>[2x]MRRETVGEFSSDDDDDILLELGTRPPRFTQIPPSSAALQTQIPTTLEVTTTTLNNKQSKNDNQLVNQLNKAQGEASMLRDKINFLNIEREKEKNIQAVKVNELQVKHLQELAKLKQELQKLEDEKKFLQMEARGKSKREVITNVKPPSTTLSTNTNTITPDSSSVAIEAKPQSPQSKKRKISDNLLKKNMVPLNPNRIIPDETSLFLESILLHQIIGADLSTIEILNRLKLDYITEFKFKNFVIAKGAPIGKSIVSLLLRCKKTLTLDRFIDTLLEDIAVLIKEISVHPNESKLAVPFLVALMYQIVQFRPSATHNLALKDCFLFICDLIRIYHHVLKVPIHESNMNLHVEPQIFQYELIDYLIISYSFDLLEGILRVLQSHPKQTYMEFFDENILKSFEFVYKLALTISYKPMVNVIFSAVEVVNIITSIILNMDNSSDLKSLISGSWWRDCITRLYALLEKEIKSGDVYNENVDTTTLHMSKYHDFFGLIRNIGDNELGGLISKLIYTDRLQSVPRVISKEDIGMDSDKFTAPIIGYKMEKWLLKLKDEVLNIFENLLMIYGDDATIVNGEMLIHSSKFLSREQALMIERYVGQDSPNLDLRCHLIEHTLTIIYRLWKDHFKQLREEQIKQVESQLIMSLWRFLVCQTETVTANEREMRDHRHLVDSLHDLTIKDQASYYEDAFEDLPEYIEEELKMQLNKRTGRIMQVKYDEKFQEMARTILESKSFDLTTLEEADSLYISMGL;>MESHVKYLDELILAIKDLNSGVDSKVQIKKVPTDPSSSQEYAKSLKILNTLIRNLKDQRRNNIMKNDTIFSKTVSALALLLEYNPFLLVMKDSNGNFEIQRLIDDFLNISVLNYDNYHRIWFMRRKLGSWCKACVEFYGKPAKFQLTAHFENTMNLYEQALTEVLLGKTELLKFYDTLKGLYILLYWFTSEYSTFGNSIAFLDSSLGFTKFDFNFQRLIRIVLYVFDSCELAALEYAEIQLKYISLVVDYVCNRTISTALDAPALVCCEQLKFVLTTMHHFLDNKYGLLDNDPTMAKGILRLYSLCISNDFSKCFVDHFPIDQWADFSQSEHFPFTQLTNKALSIVYFDLKRRSLPVEALKYDNKFNIWVYQSEPDSSLKNVTSPFDDRYKQLEKLRLLVLKKFNKTERGTLLKYRVNQLSPGFFQRAGNDFKLILNEASVSIQTCFKTNNITRLTSWTVILGRLACLESEKFSGTLPNSTKDMDNWYVCHLCDIEKTGNPFVRINPNRPEAAGKSEIFRILHSNFLSHPNIDEFSESLLSGILFSLHRIFSHFQPPKLTDGNGQINKSFKLVQKCFMNSNRYLRLLSTRIIPLFNISDSHNSEDEHTATLIKFLQSQKLPVVKENLVIAWTQLTLTTSNDVFDTLLLKLIDIFNSDDYSLRIMMTLQIKNMAKILKKTPYQLLSPILPVLLRQLGKNLVERKVGFQNLIELLGYSSKTILDIFQRYIIPYAIIQYKSDVLSEIAKIMCDGDTSLINQMKVNLLKKNSRQIFAVALVKHGLFSLDILETLFLNRAPTFDKGYITAYLPDYKTLAEITKLYKNSVTKDASDSENANMILCSLRFLITNFEKDKRHGSKYKNINNWTDDQEQAFQKKLQDNILGIFQVFSSDIHDVEGRTTYYEKLRVINGISFLIIYAPKKSIISALAQISICLQTGLGLKEVRYEAFRCWHLLVRHLNDEELSTVIDSLIAFILQKWSEFNGKLRNIVYSILDTLIKEKSDLILKLKPYT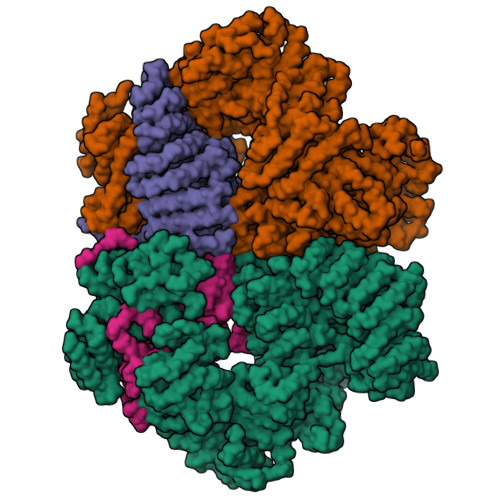TLALVGKPELGILARDGQFARMVNKIRSTTDLIPIFANNLKSSNKYVINQNLDDIEVYLRRKQTERSIDFTPKKVGQTSDITLVLGALLDTSHKFRNLDKDLCEKCAKCISMIGVLDVTKHEFKRTTYSENEVYDLNDSVQTIKFLIWVINDILVPAFWQSENPSKQLFVALVIQESLKYCGLSSESWDMNHKELYPNEAKLWEKFNSVSKTTIYPLLSSLYLAQSWKEYVPLKYPSNNFKEGYKIWVKRFTLDLLKTGTTENHPLHVFSSLIREDDGSLSNFLLPYISLDIIIKAEKGTPYADILNGIIIEFDSIFTCNLEGMNNLQVDSLRMCYESIFRVFEYCKKWATEFKQNYSKLHGTFIIKDTKTTNMLLRIDEFLRTTPSDLLAQRSLETDSFERSALYLEQCYRQNPHDKNQNGQLLKNLQITYEEIGDIDSLDGVLRTFATGNLVSKIEELQYSENWKLAQDCFNVLGKFSDDPKTTTRMLKSMYDHQLYSQIISNSSFHSSDGKISLSPDVKEWYSIGLEAANLEGNVQTLKNWVEQIESLRNIDDREVLLQYNIAKALIAISNEDPLRTQKYIHNSFRLIGTNFITSSKETTLLKKQNLLMKLHSLYDLSFLSSAKDKFEYKSNTTILDYRMERIGADFVPNHYILSMRKSFDQLKMNEQADADLGKTFFTLAQLARNNARLDIASESLMHCLERRLPQAELEFAEILWKQGENDRALKIVQEIHEKYQENSSVNARDRAAVLLKFTEWLDLSNNSASEQIIKQYQDIFQIDSKWDKPYYSIGLYYSRLLERKKAEGYITNGRFEYRAISYFLLAFEKNTAKVRENLPKVITFWLDIAAASISEAPGNRKEMLSKATEDICSHVEEALQHCPTYIWYFVLTQLLSRLLHSHQSSAQIIMHILLSLAVEYPSHILWYITALVNSNSSKRVLRGKHILEKYRQHSQNPHDLVSSALDLTKALTRVCLQDVKSITSRSGKSLEKDFKFDMNVAPSAMVVPVRKNLDIISPLESNSMRGYQPFRPVVSIIRFGSSYKVFSSLKKPKQLNIIGSDGNIYGIMCKKEDVRQDNQYMQFATTMDFLLSKDIASRKRSLGINIYSVLSLREDCGILEMVPNVVTLRSILSTKYESLKIKYSLKSLHDRWQHTAVDGKLEFYMEQVDKFPPILYQWFLENFPDPINWFNARNTYARSYAVMAMVGHILGLGDRHCENILLDIQTGKVLHVDFDCLFEKGKRLPVPEIVPFRLTPNLLDALGIIGTEGTFKKSSEVTLALMRKNEVALMNVIETIMYDRNMDHSIQKALKVLRNKIRGIDPQDGLVLSVAGQTETLIQEATSEDNLSKMYIGWLPFW[2x]> MKDRKILNEILSNTINELNLNDKKANIKIKIKPLKRKIA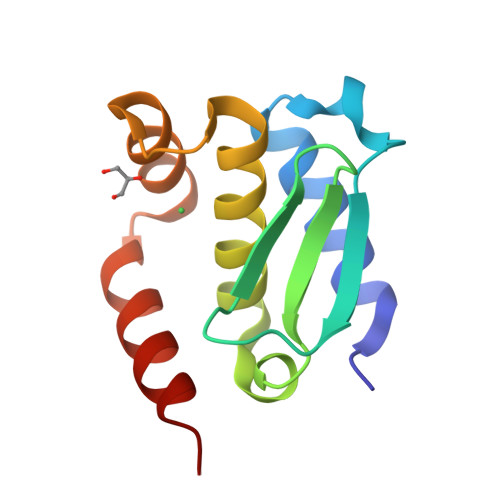SISLTNKTIYINKNILPYLSDEEIRFILAHELLHLKYGKYHINEFEEELLFLFPNKEAILINLINKLHQKK Here, we visualize, for the model phage T5, how host recognition and SE can be achieved via the interaction of different phage proteins with the same receptor in the Escherichia coli outer membrane. The receptor for phage T5 was identified as the outer membrane (OM) TonB-dependent transporter (TBDT) FhuA almost 50 y ago. To elucidate the mechanism of SE via potential TBDT structure modulation, we report here the cryo-EM structure of the FhuA–pb5 complex and the X-ray crystal structure of the FhuA–Llp complex. Our structures show that the phage lipoprotein Llp exploits the known allostery in the plug of FhuA in the opposite direction as during ferrichrome import (i.e., from the periplasmic side to the extracellular side).

Extensive screening yielded one crystal form that contained both components and had useful, anisotropic diffraction to ∼3.4 Å resolution. Adding an AF2-predicted Llp model to the MR search gave a solution that allowed building and refinement of the complete FhuA–Llp complex. Llp is bound to the periplasmic face of FhuA and makes extensive interactions with both the plug and the barrel. The total interface area is 1,640 Å2, with 14 hydrogen bonds and four salt bridges. Strikingly, several Llp residues (Ile39-Trp46) occupy space where the N-terminal switch helix of free FhuA would be, indicating that Llp has bound to a nonnative conformation of FhuA. Structural changes in the rest of the plug are less extensive but nevertheless still include backbone shifts of 3 to 4 Å downward, toward the periplasmic space. On the extracellular side, the conformational changes in FhuA–Llp relative to free FhuA are dramatic but confined to just two loops, EL7 and EL8. Both loops fold inward to completely occlude the plug domain in Llp-bound FhuA. Importantly, the effect of the EL7 and EL8 movements is that they will prevent the high-affinity binding of pb5 to FhuA because of extensive clashes with the FhuA binding loops of pb5, explaining our in vitro data with purified components and in vivo data from the literature. We propose that Llp has jammed the plug of FhuA and that any TonB pulling does not remove the phage lipoprotein from the transporter.

> SMAVEPKEDTITVTAAPAPQESAWGPAATIAARQSATGTKTDTPIQKVPQSISVVTAEEMALHQPKSVKEALSYTPGVSVGTRGASNTYDHLIIRGFAAEGQSQNNYLNGLKLQGNFYNDAVIDPYMLERAEIMRGPVSVLYGKSSPGGLLNMVSKRPTTEPLKEVQFKAGTDSLFQTGFDFSDSLDDDGVYSYRLTGLARSANAQQKGSEEQRYAIAPAFTWRPDDKTNFTFLSYFQNEPETGYYGWLPKEGTVEPLPNGKRLPTDFNEGAKNNTYSRNEKMVGYSFDHEFNDTFTVRQNLRFAENKTSQNSVYGYGVCSDPANAYSKQCAALAPADKGHYLARKYVVDDEKLQNFSVDTQLQSKFATGDIDHTLLTGVDFMRMRNDINAWFGYDDSVPLLNLYNPVNTDFDFNAKDPANSGPYRILNKQKQTGVYVQDQAQWDKVLVTLGGRYDWADQESLNRVAGTTDKRDDKQFTWRGGVNYLFDNGVTPYFSYSESFEPSSQVGKDGNIFAPSKGKQYEVGVKYVPEDRPIVVTGAVYNLTKTNNLMADPEGSFFSVEGGEIRARGVEIEAKAALSASVNVVGSYTYTDAEYTTDTTYKGNTPAQVPKHMASLWADYTFFDGPLSGLTLGTGGRYTGSSYGDPANSFKVGSYTVVDALVRYDLARVGMAGSNVALHVNNLFDREYVASCFNTYGCFWGAERQVVATATFRF;> MKKLFLAMAVVLLSACSTFGPKDIKCEAYYMQDHVKYKANVFDRKGDMFLVSPIMAYGSFWAPVSYFTEGNTCEGVFHHHHHH> SPNIEACGYSVRVMQLTLGNSTITTQEAANSVVAYGRWPEYIKDSEANPVDQPTEPDVAACRFYTLDTVTWRKESRGWWWKLPDALKDMGLFGQNMFYHYLGRAGYTVHVQCNASKFHQGALGVFAVPEMCLAGDSTTHMFTKYENANPGEKGGEFKGSFTLDTNATNPARNFCPVDYLFGSGVLAGNAFVYPHQIINLRTNNCATLVLPYVNSLSID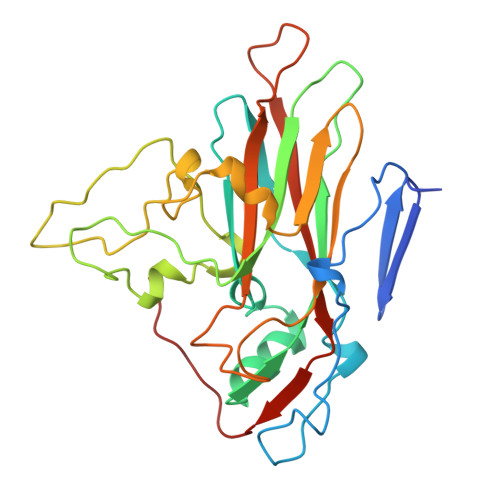SMTKHNNWGIAILPLAPLDFATESSTEIPITLTIAPMCCEFNGLRNITVPRTQ> ASYFTSVDQSSVH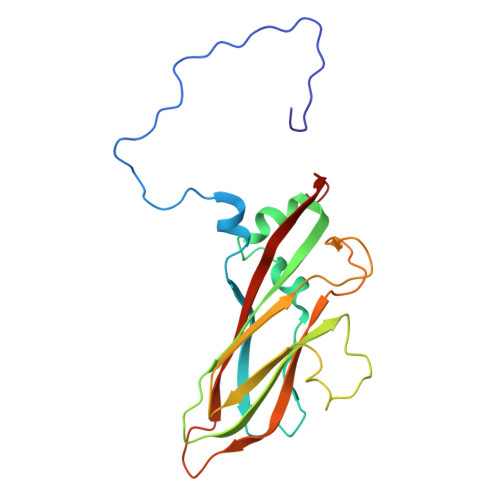TAEVGSHQIEPLKTSVDKPGSKKTQGEKFFLIHSARWLTTHALFHEVAKLDVVKLLYNEQFAVQGLLRYHTYARFGIEIQVQINPTPFQQGGLICAMVPGDQSYGSIASLTVYPHGLLNCNINNVVRIKVPFIYTRGAYHFKDPQYPVWELTIRVWSELNIGTGTSAYTSLNVLARFTDLELHGLTPLST> MQFVNKQFNYKDPVNGVDIAYIKIPNVGQMQPVKAFKIHNKIWVIPERDTFTNPEEGDLNPPPEAKQVPVSYYDSTYLSTDNEKDNYLKGVTKLFERIYSTDLGRMLLTSIVRGIPFWGGSTIDTELKVIDTNCINVIQPDGSYRSEELNLVIIGPSADIIQFECKSFGHEVLNLTRNGYGSTQYIRFSPDFTFGFEESLEVDTNPLLGAGKFATDPAVTLAHELIHAGHRLYGIAINPNRVFKVNTNAYYEMSGLEVSFEELRTFGGHDAKFIDSLQENEFRLYYYNKFKDIASTLNKAKSIVGTTASLQYMKNVFKEKYLLSEDTSGKFSVDKLKFDKLYKMLTEIYTE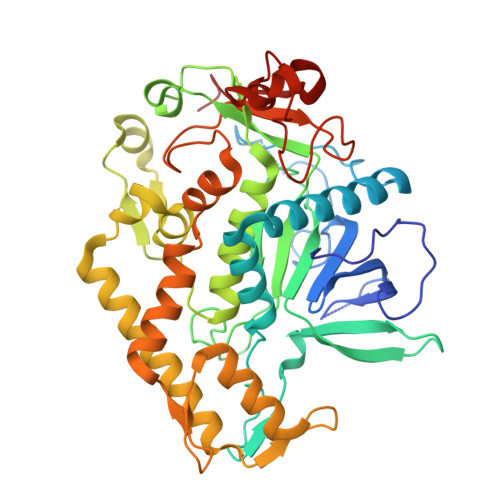DNFVKFFKVLNRKTYLNFDKAVFKINIVPKVNYTIYDGFNLRNTNLAANFNGQNTEINNMNFTKLKNFTGLFEF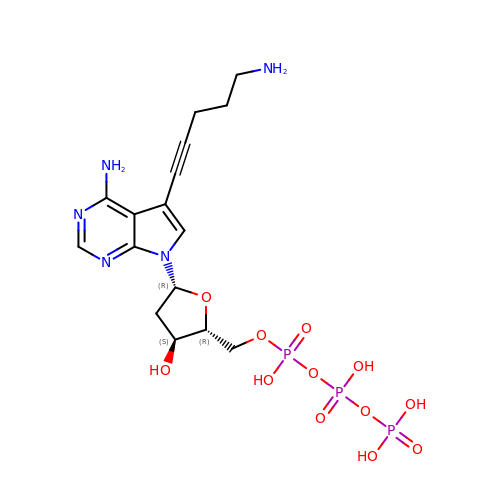5-(5-aminopent-1-yn-1-yl)-7-{2-deoxy-5-O-[(S)-hydroxy{[(S)-hydroxy(phosphonooxy)phosphoryl]oxy}phosphoryl]-beta-D-erythro-pentofuranosyl}-7H-pyrrolo[2,3-d]pyrimidin-4-amine | C16 H24 N5 O12 P3 | MCSGHAFVOBYWGE-YNEHKIRRSA-N ADENOSINE 5'-(TRIHYDROGEN DIPHOSPHATE) P'-5'-ESTER WITH 3-(AMINOCARBONYL)-4-(1-HYDROXYL-2-OXO-3-PHOSPHONOOXY-PROPYL)-1-BETA-D-RIBOFURANOSYLPYRIDINIUM 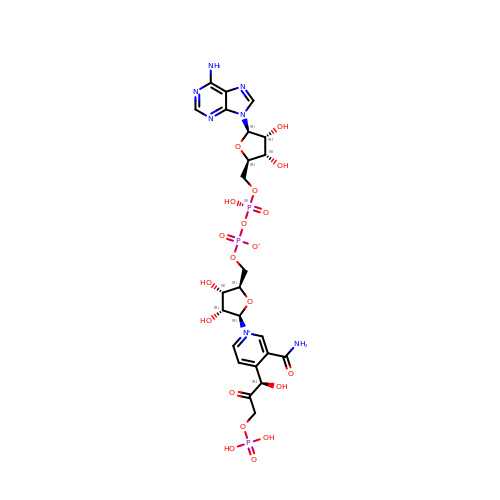INNER SALT | C24 H32 N7 O20 P3 | IVZPTIKSOMOSEU-WPIGAQFXSA-N> PISNIFAGLLFYVLSDYVTEDTGIRITRAELEKTIVEHGGKLIYNVILKRHSIGDVRLISCKTTTECKALIDRGYDILHPNWVLDCIAYKRLILIEPNYCFNVSQKMRAVAEKRVDCLGDSFENDISETKLSSLYKSQLSLPPMGELEIDSEVRRFPLFLFSNRIAYVPRRKISTEDDIIEMKIKLFGGKITDQQSLCNLIII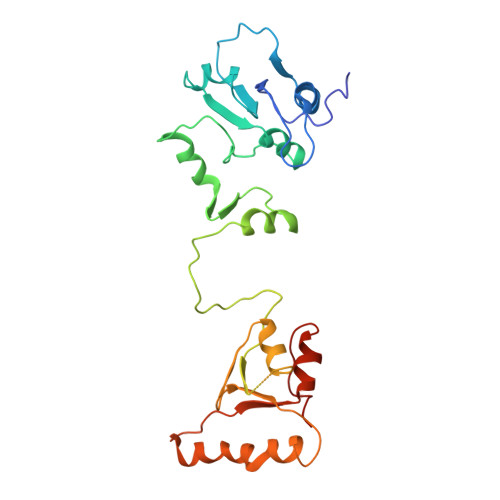PYTDPILRKDCMNEVHEKIKEQIKASDTIPKIARVVAPEWVDHSINENCQVPEEDFPVVNY> GRNGKSQSIIV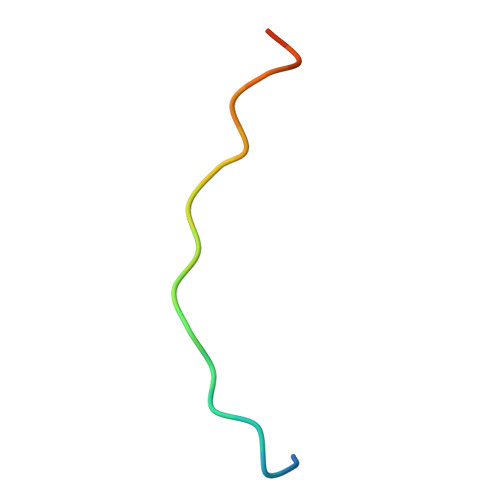GPWGDRVTN5-phosphono-D-norvaline 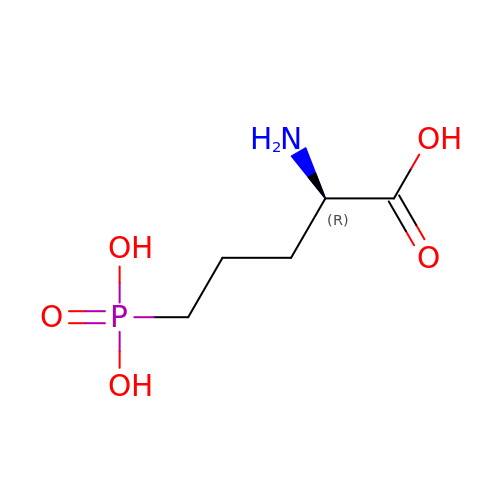| C5 H12 N O5 P | VOROEQBFPPIACJ-SCSAIBSYSA-N> AELTCTDVSGLTAEEIQMRESLQYTDHS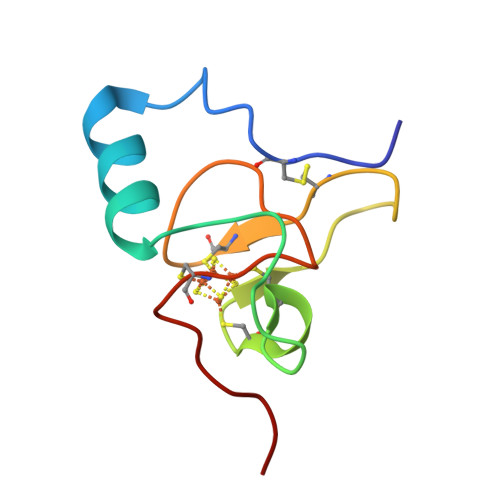PYPDKTCANCQLYVPAESPDQCGGCQLIKGPIHPNGYCTSWVQKAT>MKTSGNQDEILVIRKGWLTIN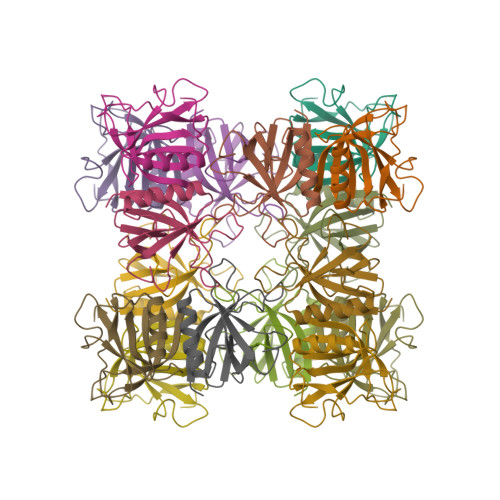NIGIMKGGSKEYWFVLTAENLSWYKDDEEKEKKYMLSVDNLKLRDVEKGFMSSKHIFALFNTEQRNVYKDYRQLELACETQEEVDSWKASFLRAGVYPERVGDK[2x]> SGIREVILCKDQDGKIGLRLKSIDNGIFVQLVQANSPASLVGLRFGDQVLQINGENCAGWSSD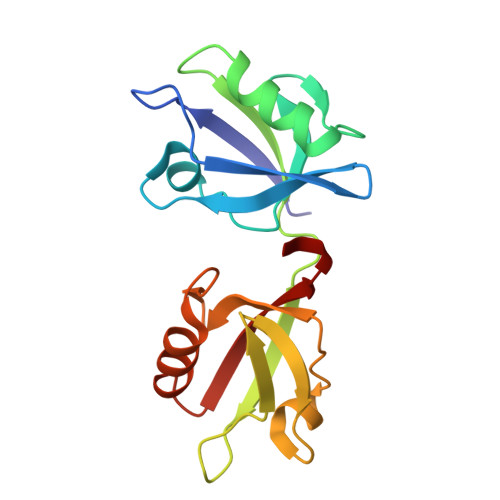KAHKVLKQAFGEKITMTIRDRPFERTITMHKDSTGHVGFIFKNGKITSIVKDSSAARNGLLTEHNICEINGQNVIGLKDSQIADILSTSGTVVTITIMPAFIF~{N}-[3-[(4~{S})-2-azanyl-6-(fluoranylmethyl)-4-methyl-1,3-oxazin-4-yl]-4-fluoranyl-phenyl]-5-cyano-pyridine-2-carboxamide 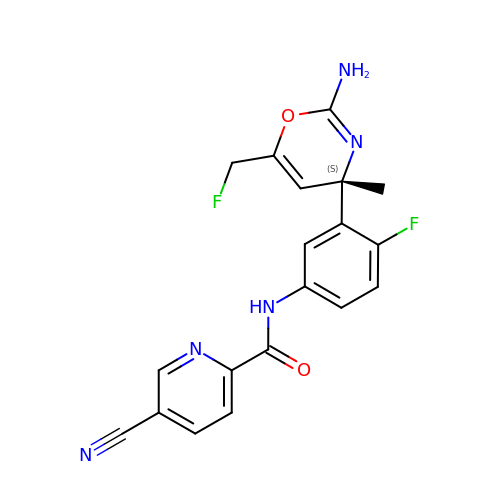| C19 H15 F2 N5 O2 | ORHZQSYKGHHDOP-IBGZPJMESA-N>MKIRTLIAMYACLLSIFIAYAYYYQQDISRIRSLQDEISSLHGKPDEKYVMVTFQSGMDYWKRCLKGFEDAAESLNVSVEYRGATQYDVNEQVTVLEQVIARKPAGIAISAINPTALTKTINKAVEEGIPVVLFDSNASGSKAFSFLGTNNYSAGVTAAHEMAKLLKSEGKVAVITSPHQLNHQERTRGFVETIYQKYPRMQVVAVKNGKGDALASKQAAMEVLNDYPD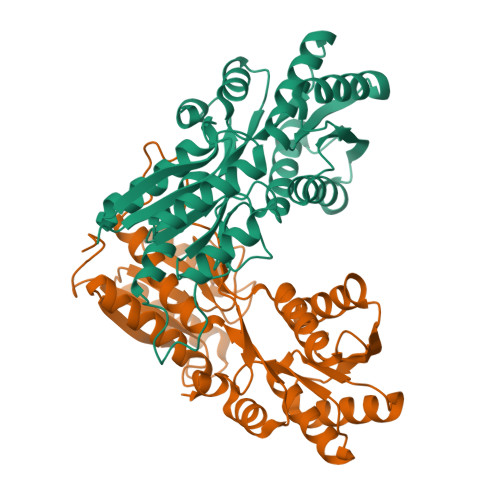VQGIFATEANGGVGMAEAVAELNKKYVKLISFDTEKQTLDLVKEGAIAATLAQGTWNMGYWSLQFLFHLHHHLTSPSRSGDALLPAYVDTGITVVTRDNVDHFYAK[2x]> GSMAVNVYSTSVTSENLSRHDMLAWVNDSL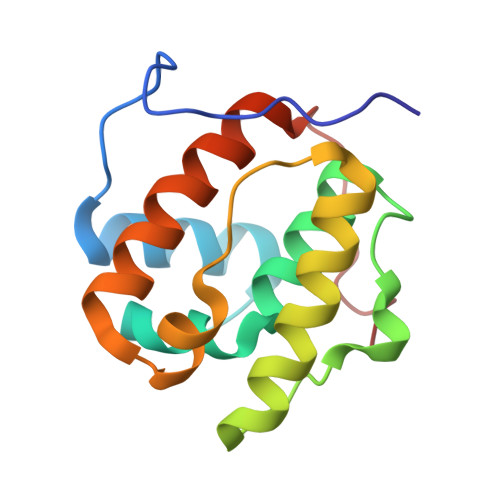HLNYTKIEQLCSGAAYCQFMDMLFPGCVHLRKVKFQAKLEHEYIHNFKVLQAAFKKMGVDKIIPVEKLVKGKFQDNFEFIQWFKKFFDANYDGKDYNPLLAR>[3x]AHCIGITDRDFIEGVHGGTWVSATLEQDKCVTVMAPDKPSLDISLETVAIDGPAEARKVCYS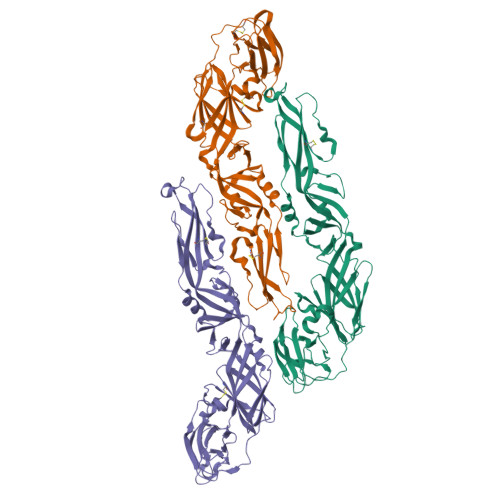AVLTNVKINDKCPSTGEAHLEEENEGDNACKRTYSDRGWGNGCGLFGKGSIVACAKFTCAKSMSLFEVDQTKIQYVIRAQLHVGAKQENWNTDIKTLKFDALSGSQEAEFTGYGRATLECQVQTAVDFSNSYIAEMEKESWIVDKQWAQDLTLPWQSGSGGVWREMHHLVEFEPPHAATIKVLALGNQEGSLKTALTGAMRVTKDTNNSKLYKLHGGHVACRVKLSALTLKGTSYKICTDKMFFVKNPTDTGHGTVVMQVKVSKGAPCRIPVIVADDLTAAINKGILVTVNPIASTNDDEVLIEVNPPFGDSYIIVGRGDSRLTYQWHK> MNQNLLVTKRDGSTERINLDKIHRVLDWAAEGLHNVSISQVELRSHIQFYDGIKTSDIHETIIKAAADLISRDAPDYQYLAARLAIFHLRKKAYGQFEPPALYDHVVKMVEMGKYDNHLLEDYTEEEFKQMDTFIDHDRDMTFSYAAVKQLEGKYLVQNRVTGEIYESAQFLYILVAACLFSNYPRETRLQYVKRFYDAVSTFKISLPTPIMSGVRTPTRQFSSCVLIECGDSLDSINATSSAIVKYVSQRAGIGINAGRIRALGSPIRGGEAFHTGCIPFYKHFQTAVKSCSQGGVRGGAATLFYPMWHLEVESLLVLKNNRGVEGNRVRHMDYGVQINKLMYTRLLKGEDITLFSPSDVPGLYDAFFADQEEFERLYTKYEKDDSIRKQRVKAVELFSLMMQERASTGRIYIQNVDHCNTHSPFDPAIAPVRQSNLCLQIALPTKPLNDVNDENGEIALCTLSAFNLGAINNLDELEELAILAVRALDALLDYQDYPIPAAKRGAMGRRTLGIGVINFAYYLAKHGKRYS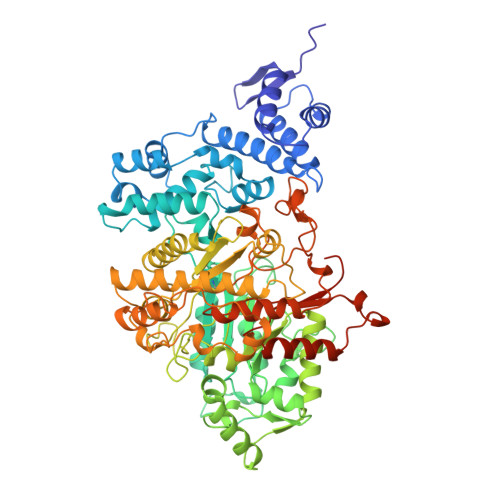DGSANNLTHKTFEAIQYYLLKASNELAKEQGACPWFNETTYAKGILPIDTYKKDLDTIANEPLHYDWEALRESIKTHGLRNSTLSALMPSETSSQISNATNGIEPPRGYVSIKASKDGILRQVVPDYEHLHDAYELLWEMPGNDGYLQLVGIMQKFIDQSISANTNYDPSRFPSGKVPMQQLLKDLLTAYKFGVKTLYYQNTRDGAEDAQDDLVPSIQDDGCESGACKI>SNAAAFKHVKSDIKIEKLNVTLNDAAKKQINNYTSQQVSNKKND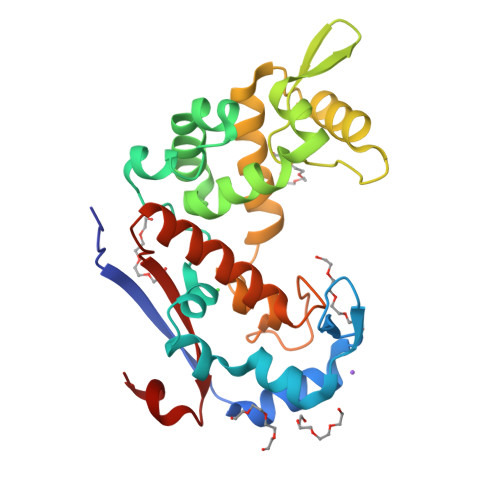AWRDASATEIKSAMDSGTFIDNEKQKYQFLDLSKYQGIDKNRIKCMLVDRPTLLKHTDDFLKAAKDKHVNEVYLISHALLETGAVKSELANGVEIDGKKYYNFYGVGALDKDPIKTGAEYAKKHGWDTPEKAISGGADFIHKHFLSSTDQNTLYSMRWNPKNPGEHQYATDIKWAESNATIIADFYKNMKTEGKYFKYFVYKDDSKHLNK[2x]> MTDRRRINGPAGATIPPVYEDSGISEVKALKIRSRPSNIIRKIYLKTGVTPSASGSAYLELETSANSGVSGLKLSCTVHGPRSLPRSSPFSPHMVVSTHVKYAPFATKQRRGY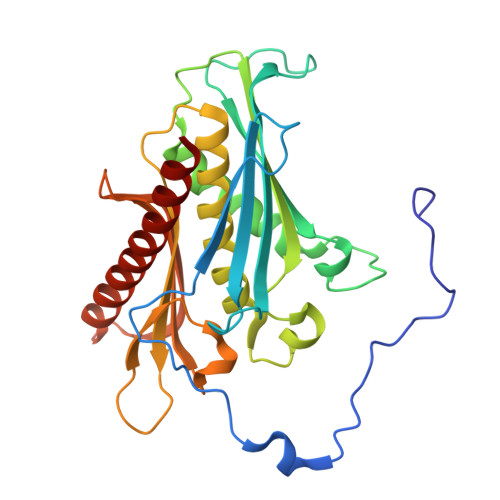LRDPTERDLGIHLEAALRGAIIADRWPKSGVDIIISIIEGDQDREASKTQGDEVWDMMNTLSGCITVASAALADAGIDCVDTVAGGVAALVQDSDGSPEIVVDPIPSEHRKILAACCVAYLPMRDEVTNLWFRGDLPASDMDLYTELVEKGIQASRSANRVLVDCLTETVG>[6x]MGIPADNLQSRAKASFDTRVAAAELALARGAVPSFANGEELLYRNSETGDPSFIGSFTKGLPHDDNGAIIDPDDFLAFVRAINSGDEKEIAALTLGPARDPETGLPIWRSDLANSLDLEVRGWENSSAGLTFDLEGPDAQSVAMPPAPVLTSPELIAEMAELYLMALGRDIEFSEFDSPKNAAFIRSAIERLNGLEWFNTPAKLGDPPAEIRRRRGEVTVGNLFRGILPGSEVGPYLSQFIIVGSKQIGSATVGNKTLVSPNAADEFDGEIAYGSITISQRVRIATPGRDFMTDLKVFLDVQDAADFRGFESYEPGARLIRTIRDLATWVHFDSLYEAYLNACLILLANGVPFDPNLPFQQEDKLDNQDVFVNFGSAHVLSLVTEVATRALKAVRYQK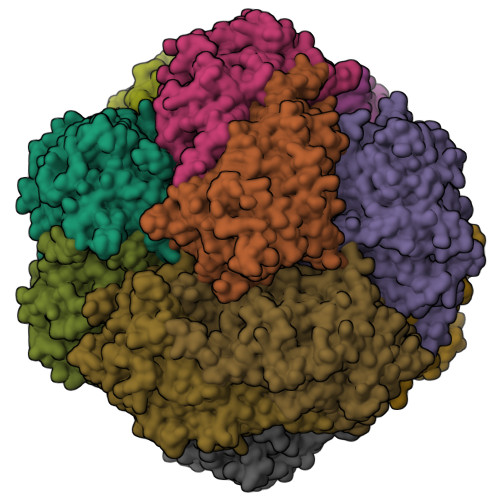FNIHRRLRPEATGGLISVNKNAFLKSESVFPEVDVLVEELSSILDDSASSNEKQNIADGDVSPGKSFLLPMAFAEGSPFHPSYGSGHAVVAGACVTILKAFFDANFQIDQVFEVDTDEDKLVKSSFPGPLTVAGELNKLADNVAIGRNMAGVHYFSDQFESLLLGEQIAIGILEEQSLTYGENFFFNLPKFDGTTIQI> MIIPALDLIGGTVVRVVRLHQGDYARLRDYGNDPLPRLQDYAAQGAGVLHLVDLTGAKDPAKRQIPLIKTLVAGVNVPVQVGGGVRTEEDVAALLKAGVARVVIASTAVKSPDVVKGWFERFGAQALVLALDVRIDEHGTKQVAVSGWQENSGVSLEQLVETYLPVGLKHVLCTDI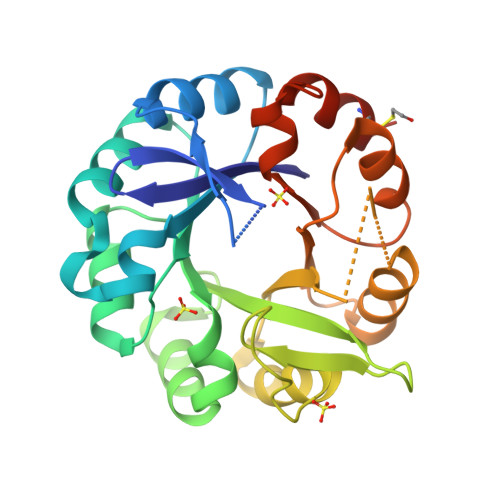SRDGTLAGSNVSLYEEVCARYPQIAFQSSGGIGDIDDIAALRGTGVRGVIVGRALLEGKFTVKEAIQCWQNVKGHHHHHH> ANGTSSAFTQIDNFSHFYDRGDHLVNGKPSFTVDQVADQLTRSGASWHDLNNDGVINLTYTFLTAPPVGYASRGLGTFSQFSALQKEQAKLSLESWADVAKVTFTEGPAARGDDGHQTFANFSASNGGAAFAYLPNSSRKGESWYLINKDYQVNKTPGEGNYGRQTLTHEIGHTLGLSHPGDYNAGNGNPTYRDAVYAEDTRAYSVMSYWSEKNTGQVFTKTGEGAYASAPLLDDIAAVQKLYGANLETRADDTVYGFNSTADRDFYSATSSTDKLIFSVWDGGGNDTLDFSGFSQNQKINLTAGSFSDVGGMTGNVSIAQGVTIENAIGGSGNDLLIGNDAANVLKGGAGNDIIYGGGGADVLWGGTGSDTFVFGAVSDSTPKAADIIKDFQSGFDKIDLTAITKLGGLNFVDAFTGHAGDAIVSYHQASNAGSLQVDFSGQGVADFL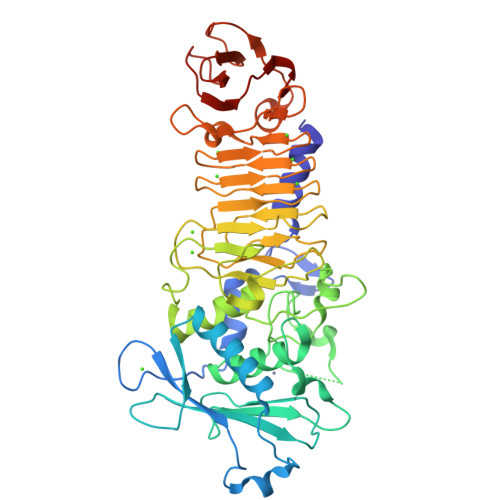VTTVGQVATYDIVA>[4x]MGSSHHHHHHSSGLVPRGSHNTRYNAADIEVLSGLDPVKRRPGMYTDTARPNHLAQEVIDNSVDEALAGHAKQIEVTLYKDGSCEVSDDGRGMPVDIHPEEKIPGVELILTRLHAGGKFNNRNYTFSGGLHGVGVSVVNALSTKVELFIKREGSEHRMEFRDGNAASKLEVVGTVGKKNTGTRLRFWADPKYFDTPKFNVRALRHLLRAKAVLCPGLTVKLHDEATGEQD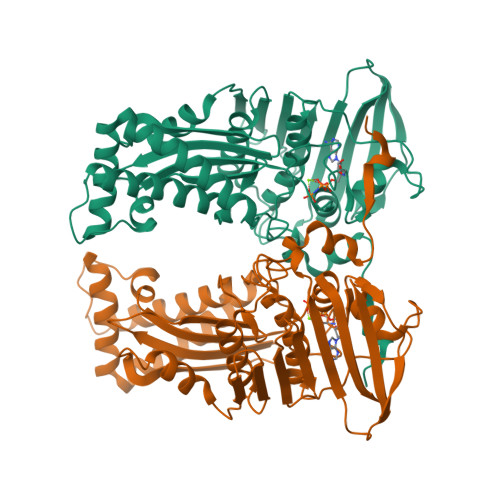SWYFENGLRDYLKGEMAEHEMLPADLFVGSLKKDTEIVDWAAGWVPEGELVQESYVNLIPTAQHGTHVNGLRSGLTDALREFCDFRNLLPRGVKLAPEDVWDRVTFVLSLKMTDPQFSGQTKERLSSRQAAGFIEGAAHDAFSLYLNQNVEIGEKIAQIAIDRASARLKTEKQIVRKK> RAITVFSPDGRLFQVEYAREAVKRGATAIGIKCKEGVILIADKRVGSKLLEADTIEKIYKIDEHICAATSGLVADARVLIDRARIEAQINRLTYDEPITVKELAKKICDFKQQYTQYGGVRPFGVSLLIAGVDEVPKLYETDPSGALLEYKATAIGMGRNAVTEFFEKEYRDDLSFDDAMVLGLVAMGLSIESELVPENIE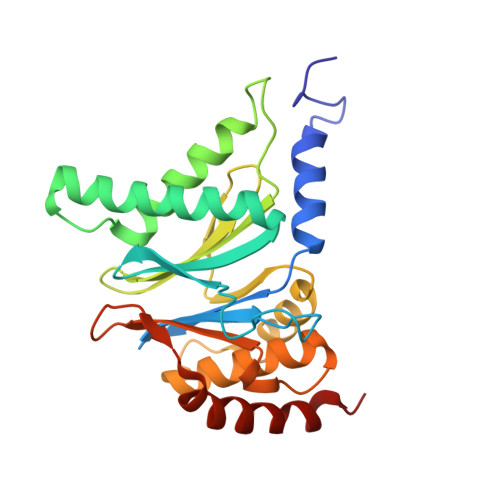VGYVKVDDRTFKEVSPEELKPYVERANERIRELLKK> GPLGSPLIGEIGPETYSDYMSAGIPLAYIFAETAEERKELSDKLKPIAEAQRGVINFGTIDAKAFGAHAGNLNLKTDKFPAFAIQEVAKNQKFPFDQEKEITFEAIKAFVDDFVAGKIEPSIKSEPIPEKQEGPVTVVVAKNYNEIVLDDTKD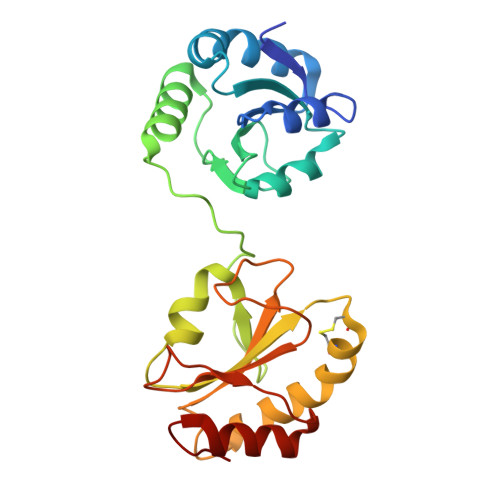VLIEFYAPWCGHCKALAPKYEELGALYAKSEFKDRVVIAKVDATANDVPDEIQGFPTIKLYPAGAKGQPVTYSGSRTVEDLIKFIAENGKYKAA> SRSLNMLGRKTC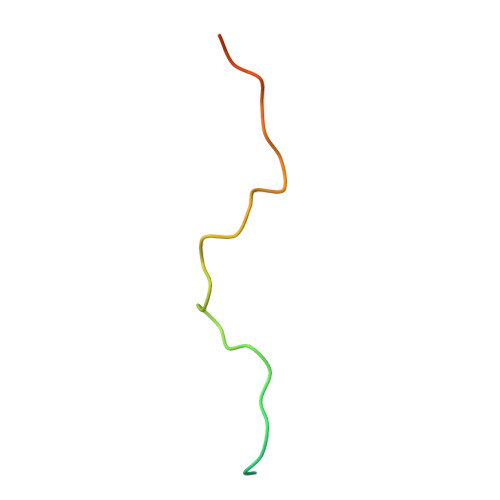LGRRVVQPGMFADYPPTKKARVLLRRMSN>FMSLFRAHLVFYRCALNLNSSYNFGFLVAMTFVLQIITGITLAFRYTSEASCAFASVQHLVREVAAGWEFRMLHATTASFVFLCILIHMTRGLYNWSYSYLTTAWMSGLVLYLLTIATAFLGYVLPWGQMSFWGATVITNLLSPIPYLVPWLLGGYYVSDVTLKRFFVLHFILPFIGCIIIVLHIFYLHLNGSSNPAGIDTALKVAFYPHMLMTDAKCLSYLIGLIFLQAAFGLMELSHPDNSIPVNRFVTPLHIVPEWYFLAYYAVLKVIPSKTGGLLVFMSSLINLGLLSEIRALNTRMLIRQQFMTRNVVSGWVIIWVYSMIFLIIIGSAIPQATYILYGRLATILYLTTGLVLCLY[2x];>[2x]MGGGGGGALNKLFPGYKDKIWMKVPVQWRQQMIQHWNKSYEKQVYSESVALNRTFQARNQLVLDRLKPSGAYRLPAVDYKRQLSRGTLVEGADFYLPTAQEQQRLARHFEPYSEQEQEERRKFRFQSISVYLAVALGASFVHDYFYQRRPVAWCLEKEPPHPPSYPFWFKSLFHSHDIPSVRRGYEVYRKVCATCHSMEQLHFRHLVGEVLPEKRVKQIAAEYDVTDGPNDQGEMYTRPGILGDAFPSPYPNEEAARYANGGAYPPDLSLITAARHFGPDYLMALLGGYRDPPEGVELRPGLYWNVWFPGNAIAMPPPLMDEMIDYEDGTPCNISQMSKDVVNFLTWATEPTADERKLYGLKCVSAIAIGTVLMTLWWRFYWAMYATRRIDFGKLKYL;>[2x]MRHLARCASRRAVKWTERDSPVANFLRSSSCCPFQLLQASRAKIQRLRTSERFRLRSAQKLAPTRFPPFTHGPLFFSLPSRLTVPSSLRSLSAFSAPLSLPFRGTMAFLSSPLFAAKASLAARVHALGCSTTSLTSPLAARALAASSLSLFSVSPRRHFSVHSHNIRPDKHELPASEVPLYYNRFDQADHPSLWQLEEEQQRKHLDQEVTDVSQLVEPVSSPHQTEGWFKRLRYWHYKETAEPTFPRTPDLSKGELAAGATVTRTSVWHDPNEPAIVSVSRFAPDNFRAVGFAENVPNPESTNSDSHPDFREYRLGPGSVDRRPFVYFMSASYFFITASMMRSFLCKWVHYWWVSRDMLAAGTTEVDLRPIQEGMTAVFKWRGKPVFVRHRTAEDIAKAQADDALIGTMKDPQLDSERCPRPQWLINIGVCTHLGCIPTDGGNYGGWFCPCHGSHYDTSGRIRLGPAPSNLELPPTVFLDDHTVKLG;>[2x]MMFRFLPRVASGASSLSVSQRRLRASFSSSLQSRGFFSAAPAAATAGVSPLARSVDAAIPEEAFNQPPTLTTTLPNGIRVATQRLPFHQTATVGVWIDSGSRYDTKETNGAAHFLEHMTFKGTKRRSRIQLEQEIENMGAHLNAYTSREQTVYYAKAFKKDIPQCVDILSDILLNSTIDEEAVQMEKHVILREMEEVERQTEEVIFDRLHTTAFRDSPLGYTILGPEENIRNMTREHILEYINRNYTSDRMVVAAAGDVDHKELTALVEKHFAGLPQPKRSKIILPTEKPFFCGSELLHRNDDMGPTAHVAVGFEGVPWKSPDAVTFMLMQAIVGSYRKHDEGIVPGKVSANATVRNVCNKMTVGCADMFSAFNTCYSDTGLFGFYAQCDEVALEHCVMEIMFGITSLSYAVTDEEVERAKAQLKTQLLGHLDSTTAVAEDIGRQMLAYGRRMPLAEFLKRLEVIDAEEVKRVAWKYLHDAEVAVAGLGPLFGMPQLINLRRATFWLRY;>MNASILFRRNAPGVSTCLRRRCLRPAALAAASASGVSTPASGVWTPAFQRTEKRFLSGAALQPKAGPAPEYRRVPFVKEDMEKVMEEVPEFKYYYVGKENTKGNVYEGIPLDQSILEPADLRDYVPPHSNIQYSKLDNGLRIASMDRGGLTASLGLFVHAGTRFEDVTNFGVTHMIQNLAFASTAHLSLLRTVKTIEVLGANAGCVVGREHLVYSAECLRSHMPLLVPMLTGNVLFPRFLPWELKACKEKLIMARKRLEHMPDQMVSELLHTTAWHNNTLGHKLHCTERSLGHYNPDVIRHYMLQHFSPENMVFVGVNVNHDELCTWLMRAFVDYNAIPPSKRTVASPVYTGGDVRLETPSPHAHMAIAFETPGGWNGGDLVAYSVLQTILGGGGAFSTGGPGKGMYTRLYLNVLNQNEWVESAMAFNTQYTDSGIFGLYMLADPTKSANAVKVMAEQFGKMGSVTKEELQRAKNSLKSSIFMNLECRGIVMEDVGRQLLMSNRVISPQEFCTAIDAVTEADIKRVVDAMYKKPPTVVAYGDVSTVPHYEEVRAALRAAGVGK[2x];>MSYPYYCEFFVKFPNYIPPKDPAERLVDPRQKLEPGCTARCSLWVNEYDACTKRVRARTDNKGNCSGQYEELHVCIDRCVAKDIFKYLK[2x];>MAQFHREIGKLFASYSNKITANSPVQYVPSPPTKGKVRRALSSALMPVWFKFFRGPLDRWNLAVMAKYLRDHGLMYDDLYSDKEPVFARALELLPPDIQAARFRRLMRGTYLNHLRLYLPVHEQNYDPFIPYMAPYVEEAKFQLQEEEELLGYHMWEGVWYSGGVTGFGDKEPGEHFLVALPNLYGAGGSPMQAGGKHFSSHAASAARARLATLAQKRLEEAMQQRERQSVSQN[2x];>[2x]MAASRLCQYLAGRGQTGLLSLSAPRLGAPKFERKMLGSYPVSPEFEMVWRDRLTAHGGYIQQTISPYQLKFIYPFWHTFFARCWCKCSAYAWPWVWPGLITFGLVKKMNHDVEEDIRDHYWY;>MHFSGVFLRTSRVFLASESSAAGSKVAKSLPGIRFGNPWRDDYPEWIWKSLRVSRKDKDMFAPFFKLLNATKLYEYCLKDNRRYCMFVMGVGLVSSWMWSEWWNSVWRRINKGKLYNDVPYVYPEEDE[2x];>MSRAVYAKLWASTAQYTQRRHYAWYQIWSRVIPWSVPWGIFAMWMVFPAMPVEYRQALTFGIWQKPNIGTHGPDPADAKK[2x];>MATHNCLRQTAAQMLGQNANVFRFFSKSAPSRPSGNVALESVKNAAVAETETFAGRANVAAGTGKLEGSLLPPPHIPGIRRAPREPASPKMAGMEGRMPVRLPPEGSRFRQYVDPRADVYFPLTAVLVTLGPLYMFSKAFF[2x];>MNCPNLPAPEEFVVPVFSAGPPVGKNCFHCGIRLRRGHSSPTYSFPPYCVTMSYGNGTVLMPIVRRVFIGALVGIYAYAATDVVLIPGYAQLMQKWKKGSSTPAHGGGH[2x]

CIII (cytochrome bc1 complex) plays a crucial role in electron transfer and proton pumping. The pumping of protons into the cristae lumen occurs via the Q-cycle, which involves sequential ubiquinol oxidation and ubiquinone reduction. Both reactions occur in specific quinone binding sites within the cytochrome b (Cyt-b) subunit, called Qo (oxidation) and Qi (reduction), which are essential for catalytic activity. Likewise, in the apicomplexan mETC, complex III2 (CIII) is the primary target for antiparasitic drugs.

To reveal its binding mechanism at high resolution, we affinity-purified the T. gondii CIII embedded in amphipols via the 3xFLAG-tagged Rieske subunit, inhibited by ELQ-300 only, and determined its cryo-EM structure to 1.8 Å resolution. Surprisingly, the C2-symmetric CIII structure contains two bound ELQ-300 molecules per Cyt-b monomer, one at the Qi site and, unexpectedly, another in the central cavity of the Qo channel. In the Qi pocket, ELQ-300 displays an unexpected binding mode, which is well supported by our cryo-EM density. The 4-(1H)-quinolone group is pinned by hydrogen bonds with H197 and D223, interacting with ketone and amino groups of the ligand at N–O distances of 3.0 Å, respectively. The ketone group of ELQ-300 also interacts with the heme bH propionate group via an ordered water. Owing to the fixed orientation of the quinolone group in our T. gondii structure, the diarylether group in position-2 extends toward helix D (on the matrix side), which is markedly different from the binding pose observed in the bovine homolog, in which quinolones with both 2- or 3-diaryl-groups extend in the opposite direction, toward helix A (in the lumen side). In our T. gondii structure, the orientation of the first aryl group is determined by the adjacent I193 on helix D, leading to a 63° angle between the aryl and quinolone planes. The peripheral trifluoro-methoxy-phenoxy group displays flexibility and adopts two distinct conformations. Conformer A makes contacts along helix D with I189, V190 and I193, whereas through a rotation around the ether bond, conformer B extends toward helix a to interact with a set of hydrophobic residues. Thus, our structure reveals an unexpected binding mode of the ELQ-300 in the apicomplexan Qi site, which differs markedly from previously determined structures of the inhibited mammalian CIII and provides an accurate molecular model for developing antimalarial inhibitors.> MGNASSIVQTINVTGDGNVFKPSAETSSTAVPSLSLSPGMLNPGGVPWIAVGDETSVTSPGALRRMTSKDIPETAIINTDNSSGAVPSESALVPYIDEPLVVVTEHAITNFTKAEMALEFNREFLDKMRVLSVSPKYSDLLTYVDCYVGVSARQALNNFQKQVPVITPTRQTMYVDSIQAALKALEKWEIDLRVAQTLLPTNVPIGEVSCPMQSVVKLLDDQLPDDSLIRRYPKEAAVALAKRNGGIQWMDVSEGTVMNEAVNAVAASALAPSASAPPLEEKSKLTEQAMDLVTAAEPEIIASLAPVPAPVFAIPPKPADYNVRTLRIDEATWLRMIPKSMNTPFQIQVTDNTGTNWHLNLRGGTRVVNLDQIAPMRFVLDLGGKSYKETSWDPNGKKVGFIVFQSKIPFELWTAASQIGQATVVNYVQLYAEDSSFTAQSIIATTSLAYNYEPEQLNKTDPEMNYYLLATFIDSAAITPTNMTQPDVWDALLTMSPLSAGEVTVKGAVVSEVVPADLIGSYTPESLNASLPNDAARCMIDRASKIAEAIKIDDDAGPDEYS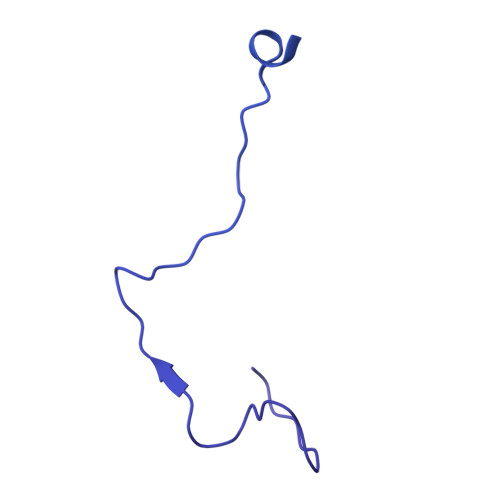PNSVPIQGQLAISQLETGYGVRIFNPKGILSKIASRAMQAFIGDPSTIITQAAPVLSDKNNWIALAQGVKTSLRTKSLSAGVKTAVSKLSSSESIQNWTQGFLDKVSAHFPAPKPDCPTSGDSGESSNRRVKRDSYAGVVKRGYTR> VEPSGHAADRIARLPGQPAVDFDMYSGYITVDEGAGRSLFYLLQEAPEDAQPAPLVLWLNGGPGCSSVAYGASEELGAFRVKPRGAGLVLNEYRWNKVANVLFLDSPAGVGFSYTNTSSDIYTSGDNRTAHDSYAFLAKWFERFPHYKYRDFYIAGESYAGHYVPELSQLVHRSKNPVINLKGFMVGNGLIDDYHDYVGTFEFWWNHGIVSDDTYRRLKEACLHDSFIHPSPACDAATDVATAEQGNIDMYSLYTPVCNITSS;> TGSYDPCTERYSTAYYNRRDVQMALHANVTGAMNYTWATCSDTINTHWHDAPRSMLPIYRELIAAGLRIWVFSGDTDAVVPLTATRYSIGALGLPTTTSWYPWYDDQEVGGWSQV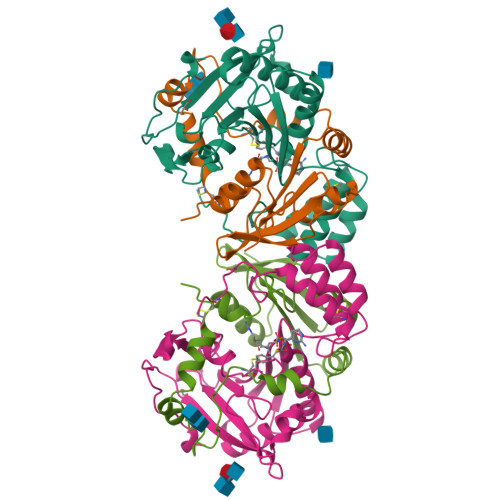YKGLTLVSVRGAGHEVPLHRPRQALVLFQYFLQGKPMPGQTKNAT> E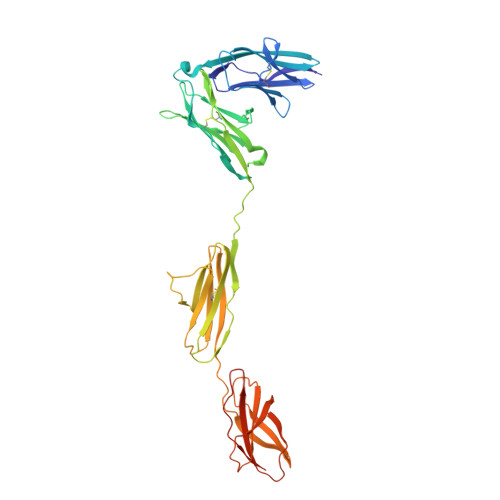TPPRFTRTPVDQTGVSGGVASFICQATGDPRPKIVWNKKGKKVSNQRFEVIEFDDGSGSVLRIQPLRTPRDEAIYECVASNNVGEISVSTRLTVLREDQIPRGFPTIDMGPQLKVVERTRTATMLCAASGNPDPEITWFKDFLPVDTSNNNGRIKQLRSESIGGTPIRGALQIEQSEESDQGKYECVATNSAGTRYSAPANLYVRELREVRRVPPRFSIPPTNHEIMPGGSVNITCVAVGSPMPYVKWMLGAEDLTPEDDMPIGRNVLELNDVRQSANYTCVAMSTLGVIEAIAQITVKALPKPPGTPVVTESTATSITLTWDSGNPEPVSYYIIQHKPKNSEEPYKEIDGIATTRYSVAGLSPYSDYEFRVVAVNNIGRGPASEPVLTQKHHHHHH> YDPDQYSIEADKKFKYSVKLSDYPTLQDAASAAVDGLLIDRDYNFYGGETVDFGGKVLTIECKAKFIGDGNLIFTKLGKGSRIAGVFMESTTTPWVIKPWTDDNQWLTDAAAVVATLKQSKTDGYQPTVSDYVKFPGIETLLPPNAKGQNITSTLEIRECIGVEVHRASGLMAGFLFRGCHFCKMVDANNPSGGKDGIITFENLSGDWGKGNYVIGGRTSYGSVSSAQFLRNNGGFERDGGVIGFTSYRAG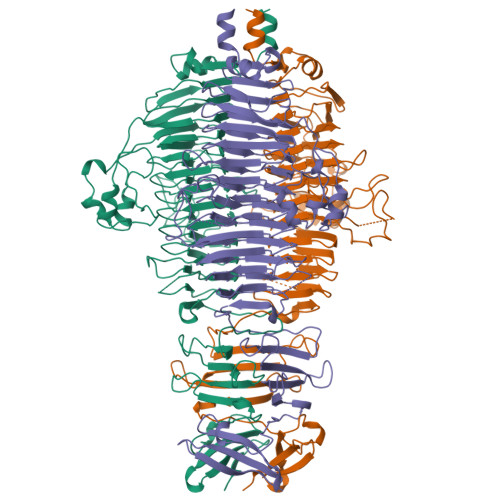ESGVKTWQGTVGSTTSRNYNLQFRDSVVIYPVADGFDLGADTDMNPELDRPGDYPITQYPLHQLPLNHLIDNLLVRGALGVGFGMDGKGMYVSNITVEDCAGSGAYLLTHESVFTNIAIIDTNTKDFQANQIYISGACRVNGLRLIGIRSTDGQSLTIDAPNSTVSGITGMVDPSRINVANLAEEGLGNIRANSFGYDSAAIKLRIHKLSKTLDSGALYSHINGGAGSGSAYTQLTAISGSTPDAVSLKVNHKDCRGAEIPFVPDIASDDFIKDSSCFLPYWENNSTSLKALVKKPNGELVRLTLATL Left-handed G4s are characterized by the anticlockwise rotation of the backbone in its helical progression. They have several unique and distinct structural features, such as: (i) ability to form stable four-layered and bi-layered dimeric structures, (ii) stacking of thymine loops with the outer tetrads (T-capping) and (iii) the local sugar orientation of each base is almost perpendicular to the overall backbone progression giving rise to the ‘twisted’ backbone. Bulges are important structural elements of G4s, which form as protrusions of bases from the G-tetrad core. Here we report on the ability of the 12-nt sequence GTGGTGGTGGTG called LHG4motif to drive several DNA sequences towards left-handed G4s with bulges.

The sequence 1xBulge-LHG4motif-TT with two additional thymines (TT) at the 3′-end was crystallized. Addition of 3′-end thymines (TT) has improved the crystal packing to provide high-quality X-ray diffraction data. 1xBulge-LHG4motif-TT was found to crystallize in the P21 space group with high-resolution diffraction to 1.18 Å. The crystal structure of 1xBulge-LHG4motif-TT features a four-layered unimolecular G4 structure separated into two blocks connected by a thymine linker. Each block has parallel left-handed backbone progression similar to the previously reported left-handed G4 structure of Z-G4 (46). The 5′-5′ stacking interface between guanine bases in successive blocks is in the opposite-polarity mode with partial 5/6-membered ring overlap. The upper block has three T-capping residues, while the lower block has four. The thymine residue T5 forming a bulge between the G4 and G6 stacked guanines, projecting out of the G-tetrad core, yielding the first left-handed G4 structure accommodating a bulge. The overhang additional 3′-thymines (TT) stack on the capping thymines, while a spermine molecule (from the crystallization solution) stacks over the outer tetrad in each block squeezing itself between the capping thymines. The accommodation of spermine stacking over the tetrads despite the presence of capping thymines establishes the possibility of ligands binding to left-handed G4s.

> GGTGTGTGGTGGTGTGGTGGTGGTGTT> GAMGPTSNDACLSIVHSLMCHRQGGESETFAKRAIESLVKKLK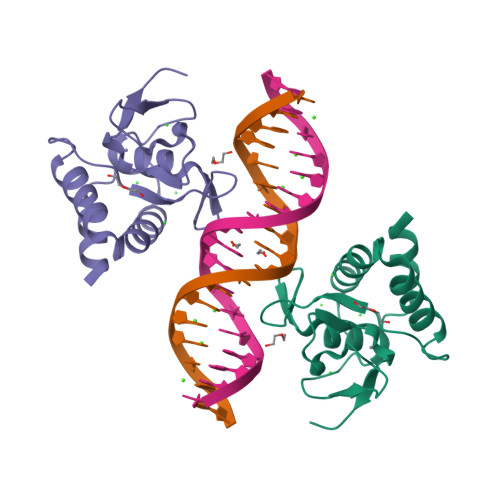EKKDELDSLITAITTNGAHPSKCVTIQRTLDGRLQVAGRKGFPHVIYARLWRWPDLHKNELKHVKYCQYAFDLKCDSVCVNPYHYERVVSPG>[2x]MVL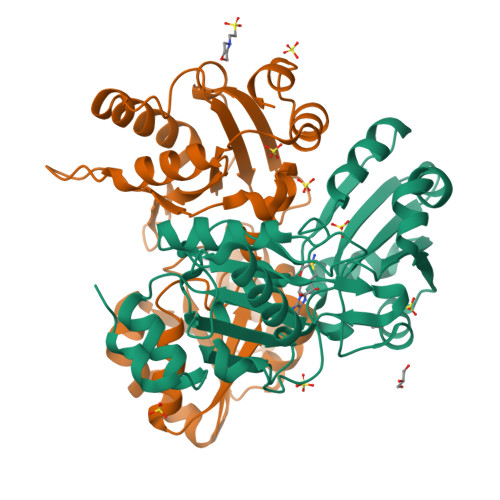YFIGLGLYDERDITVKGLEIAKKCDYVFAEFYTSLMAGTTLGRIQKLIGKEIRVLSREDVELNFENIVLPLAKENDVAFLTPGDPLVATTHAELRIRAKRAGVESYVIHAPSIYSAVGITGLHIYKFGKSATVAYPRGNWFPTSYYDVIKENAERGLHTLLFLDIKAEKRMYMTANEAMELLLKVEDMKKGGVFTDDTLVVVLARAGSLNPTIRAGYVKDLIREDFGDPPHILIVPGKLHIVEAEYLVEIAGAPREILRVNV Further, the in vitro assay confirmed that NasF5053 could produce NAS-C (47.4%), Asp-A (44.4%), as well as a minor product NAS-B (8.2%) (trace I). NasF5053 adopts the prism-like fold characteristic for P450s, consisting of a large domain of 10-helices (C-L) and a small domain of four α-helices (A, B, B’, and K’) and three β-sheets (strands β1-1 to 4, β2-1 to 2, and β3-1 to 2). Our systematic mutagenesis studies on the promiscuous NasF5053 and the versatile NascB identified four key resides, Q65, A86, S284, and V288, which play critical roles in controlling product regio-configurations and stereo-configurations. To obtain insights into the structural basis for regio-specificity, stereo-specificity, and chemical versatility, we further determined high-resolution crystal structures of wild-type NasF5053 in its substrate-free and substrate-bound form, and of two NasF5053 mutants (Q65I-A86G and S284A-V288A) in their substrate-bound forms.

Comparisons among the three substrate-bound structures showed that all substrate-interacting residues, the heme, and the two substrates superimpose well (RMSD in this region between any two structures <0.26 Å), except for the mutated residues and the adjacent residues such as K289 and I87. The plotting of the spectral variation as a function of cWL-PL concentration is fitting to a rectangular hyperbola curve, yielding a binding constant of 11.6 ± 2.1 µM for the interaction between cWL-PL and wild-type NasF5053, 25.6 ± 1.0 µM for cWL-PL with NasF5053-Q65I-A86G and 4.81 ± 0.26 µM for cWL-PL with NasF5053-S284A-V288A. The mutations of S284-V288 regulate regio-selectivity and stereo-selectivity by adjusting the relative positions of the two substrates and their conformations. Given that S284 and V288 contribute to lining the binding pocket for cWL-PL-E, mutations to less bulky Ala residues create space for cWL-PL-E to move towards the heme. This movement disturbs the interactions with the cWL-PL-U radical, and in turn pushes away the DKP and propyl rings of cWL-PL-U towards αI (orange sticks in Fig. 4b). MD also shows that the probability of the C2-N10 distance in the wild-type protein being >4 Å or <4 Å is almost equal, which means that native NasF5053 could catalyze the formation of the products either requiring or escaping intramolecular cyclization. In the S284-V288 mutant, however, this distance is fixed between 3.0 and 3.5 Å, making intramolecular cyclization inevitable.

> GSTLTYPFHDWSQELSPRYAQLRASDAPVCPVVSEGTGDPLWLVTRYATAVKLLEDSRFSSEAAQASGAPRQEPVELRAPGTRGDAIAMLREAGLRSVLADGLGPRAVRRHQGWINDLAETLMSELASREGTFDLAADFVEPLSSALVSRTLLGELSADERDLLAHCADTGLRFCGVTHEEQVHAFTQMHEFFLEHARRLAGTPGEHLLKLIAEAPVDQGPLSDEALAEAGSLLVVAGFPTSSGFLCGALLTLLRHPDAVQELHAHPERVPSAVEELLRYTPLATGSAKRMATEDLEIDGVRIKAGEVVMVSLEAVNHDPDAFEDPDVFRPGREGPMHFGFGRGRHFCPGNRLARCVIEATVRAVARRPGLRLAVAPEEISWHEGLFFRRPRAIPATW~{N}-[(3-chlorophenyl)methyl]-1-(1~{H}-indol-3-ylmethyl)piperidin-4-amine 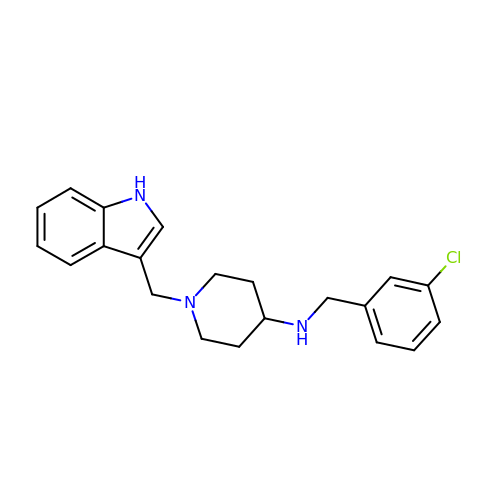| C21 H24 Cl N3 | ZBFRXMWMJAMISF-UHFFFAOYSA-N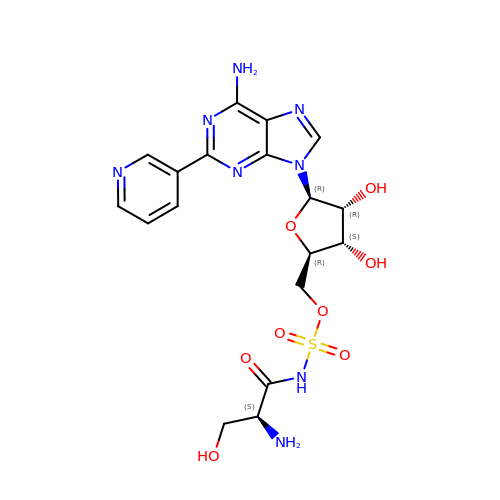[(2~{R},3~{S},4~{R},5~{R})-5-(6-azanyl-2-pyridin-3-yl-purin-9-yl)-3,4-bis(oxidanyl)oxolan-2-yl]methyl ~{N}-[(2~{S})-2-azanyl-3-oxidanyl-propanoyl]sulfamate | C18 H22 N8 O8 S | AJLUWRJYNKUFKX-OBXKABKQSA-N> FADDHAMSPDMKLLAGASNWVNQSGSVAQFVFTPSPTQPQTYEVSGNYINNAQGTGCKGTPYPLSGAYYSGNQIISFSVVWSNASANCQSATGWTGYFDFSGSQAVLKTDWNLAFYSGSTPAIQQ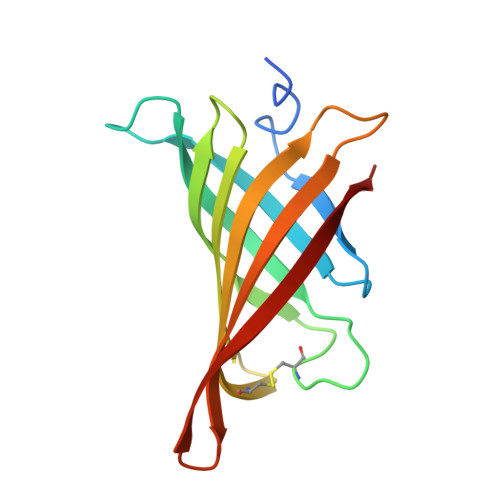GQDDFMQSV> GMSDVAETLDPLRLPLQGERLIEASAGTGKTFTIAALYLRLLLGLGGSAAFPRPLTVEELLVVTFTEAATAELRGRIRSNIHELRIACLRETTDNPLYERLLEEIDDKAQAAQWLLLAERQMDEAAVFTIHGFCQRMLNLNAFESGMLFEQQLIEDESLLRYQACADFWRRHCYPLPREIAQVVFETWKGPQALLRDINRYLQGEAPVIKAPPPDDETLASRHAQIVARIDTVKQQWRDAVGELDALIESSGIDRRKFNRSNQAKWIDKISAWAEEETNSYQLPESLEKFSQRFLEDRTKAGGETPRHPLFEAIDQLLAEPLSIRDLVITRALAEIRETVAREKRRRGELGFDDMLSRLDSALRSESGEVLAAAIRTRFPVAMIDEFQDTDPQQYRIFRRIWHHQPETALLLIGDPKQAIYAFRGADIFTYMKARSEVHAHYTLDTNWRSAPGMVNSVNKLFSQTDDAFMFREIPFIPVKSAGKNQALRFVFKGETQPAMKMWLMEGESCGVGDYQSTMAQVCAAQIRDWLQAGQRGEALLMNGDDARPVRASDISVLVRSRQEAAQVRDALTLLEIPSVYLSNRDSVFETLEAQEMLWLLQAVMTPERENTLRSALATSMMGLNALDIETLNNDEHAWDVVVEEFDGYRQIWRKRGVMPMLRALMSARNIAENLLATAGGERRLTDILHISELLQEAGTQLESEHALVRWLSQHILEPDSNASSQQMRLESDKHLVQIVTIHKSKGLEYPLVWLPFITNFRVQEQAFYHDRHSFEAVLDLNAAPESVDLAEAERLAEDLRLLYVALTRSVWHCSLGVAPLVRRRGDKKGDTDVHQSALGRLLQKGEPQDAAGLRTCIEALCDDDIAWQTAQTGDNQPWQVNDVSTAELNAKTLQRLPGDNWRVTSYSGLQQRGHGIAQDLMPRLDVDAAGVASVVEEPTLTPHQFPRGASPGTFLHSLFEDLDFTQPVDPNWVREKLELGGFESQWEPVLTEWITAVLQAPLNETGVSLSQLSARNKQVEMEFYLPISEPLIASQLDTLIRQFDPLSAGCPPLEFMQVRGMLKGFIDLVFRHEGRYYLLDYKSNWLGEDSSAYTQQAMAAAMQAHRYDLQY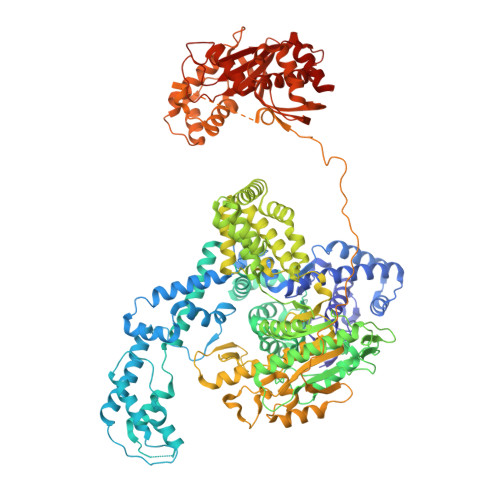QLYTLALHRYLRHRIADYDYEHHFGGVIYLFLRGVDKEHPQQGIYTTRPNAGLIALMDEMFAGMTLEEA During cell division, these autolysins are responsible for splitting the equatorial septum between two dividing daughter cells. The highly similar AtlA and AtlE proteins consist of a signal peptide, a pro-peptide, a catalytic domain with N-acetylmuramyl-L-alanine amidase activity, three repeats (R1-R3), and a C-terminal catalytic domain with N-acetylglucosaminidase activity. The catalytic domain, referred to as AmiE in S. epidermidis and AmiA in S. aureus, cleaves the amide bond between the lactyl moiety of N-acetylmuramic acid (MurNAc) and L-alanine in the PGN structure.

To provide a structural basis of autolysis function in S. epidermidis, we crystallized the catalytically active AmiE domain and solved its structure at 1.7 Å resolution. The AmiE protein adopts a globular, mixed α/β fold, with a six-stranded, central β-sheet surrounded by seven α-helices. The rear of the β-sheet packs against helices α4 and α7 and is shielded from solvent, while its front forms the bottom of a recessed area that is largely exposed and solvent-accessible. The recessed area, measuring about 28 Å by 10 Å, is walled off by helices α2, α3, α5, and several loops. Located at the center of the recessed area is a zinc ion that is held in place with contacts to side chains of residues H60 (β2), H165 (α5) and D179 (α5-α6 loop). The tetrahedral coordination sphere of zinc is completed by a water molecule, an arrangement often seen in the active sites of zinc-dependent metalloenzymes. The conserved residues delineate a groove that runs along the recessed area, extending from the zinc ion to both the top and the bottom of the domain. The shape of the groove and its high degree of conservation indicate that it is the site of interaction with the PGN substrate. Moreover, the presence of zinc at the center of the groove suggests that AmiE functions as a zinc-dependent amidase. Residues E119 and H177, which are near the zinc ion but do not contact it, are likely to be involved in catalysis by facilitating a water-mediated nucleophilic attack at the peptide bond and stabilizing the transition state, as shown in Figure 3B. A DALI analysis shows that the closest structural homolog of AmiE is the N-terminal domain of PlyL, a prophage endolysin encoded by the Bacillus anthracis genome (Z-score = 18.4, rmsd = 2.1).

>[2x]VSSQKTSSLPKYTPKVNSSINNYIRKKNMKAPRIEEDYTSYFPKYGYRNGVGRPEGIVVHDTANDNSTIDGEIAFMKRNYTNAFVHAFVDGNRIIETAPTDYLSWGAGPYGNQRFINVEIVHTHDYDSFARSMNNYADYAATQLQYYNLKPDSAENDGRGTVWTHAAISNFLGGTDHADPHQYLRSHNYSYAELYDLIYEKYLIKTKQVAPWG DNA ligase IV (LigIV) plays a major role in ligation of double-strand break (DSB) repair through nonhomologous end joining (NHEJ). DNA ligases I (LigI), III (LigIII), and LigIV share a common architecture of the catalytic region including the DNA-binding domain (DBD), the nucleotidyltransferase domain (NTase), and the OB-fold domain (OBD). NTase has the ATP-grasp fold and is a member of the glutathione synthetase ATP-binding domain-like superfamily, comprising two subdomains that have the RAGNYA fold and the phosphatidylinositol phosphate kinase (PIPK) C-terminal-like fold. In the DNA-bound form of DNA ligases (Pascal et al., 2004; Nair et al., 2007; Cotner-Gohara et al., 2010), the subdomain with the RAGNYA fold is located at the 5′ end of a DNA nick (here called NTase-5), while the second subdomain lies at the 3′ end of a DNA nick (here called NTase-3).

We crystallized a subdomain of NTase (NTase-3) of human LigIV and solved the structure at the resolution of 2.9 Å using SAD and SIRAS methods (see Experimental Procedures for the details). The structure revealed an overall architecture of the NTase-3 of LigIV that is similar to that of LigI (Pascal et al., 2004) and LigIII (Cotner-Gohara et al., 2010). LigIV has a six amino acid insert, which is relatively acidic, between β2 and 310 defined by residues of low conservation across species. The relative arrangement of motifs I, III, and IIIa resembles that of the other human DNA ligases, suggesting that LigIV carries out DNA ligation in a conventional manner. NTase-3 of DNA ligases has a DNA-binding region and loop immediately after β1 (D1) and the other between β3 and β4. The latter is mostly disordered in the crystals studied here. With the exception of a few organisms in which histidines and phenylalanines are located in the equivalent position (data not shown), Y298 is conserved among LigIVs suggesting that this residue may play a role in DNA binding. R278, Q280, and H282, mutations of which cause LIG4 syndrome, are located on β1 in the same way as the equivalent residues of LigI and LigIII. Some organisms have phenylalanine instead of tyrosine at this position. This tyrosine residue forms a part of the hydrophobic core of the NTase-3 domain and a hydrogen bond with H316, suggesting that the mouse Y288C substitution impairs the stability of NTase-3.

> FYIETKLDGERMQMHKDGDVYKYFSRNGYNYTDQFGASPTEGSLTPFIHNAFKADIQICILDGEMMAYNPNTQTFMQKGTKFDIKRMVEDSDLQTCYCVFDVLMVNNKKLGHETLRKRYEILSSIFTPIPGRIEIVQKT>[2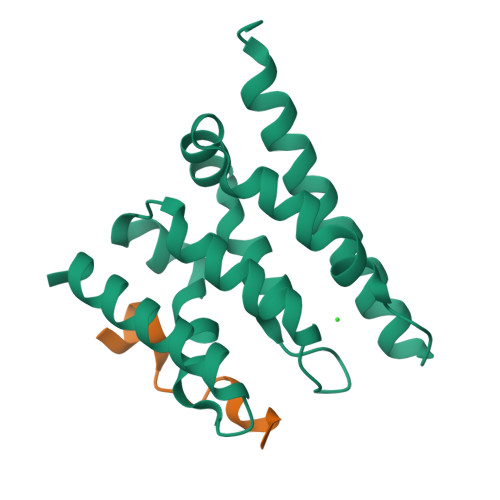x]MDPGTVLEISRSLKKRMQDILKKDNANNLEGRPATGKIENVEEISDILMSKALQESLLDEGILDEIKGWLEPLPDKSMPNIKIRKRLLDVLKTMKIHKEHLVTSGVGKIVYFYSINPKESKEVRASAKALVQKWTNEVFKPEGGD;>[2x]GSHMFFEIFGTGEEYRYVLESDP>[3x]SNATLRIAAMPALANGLLPRFLAQFIRDRPNLQVSLMGL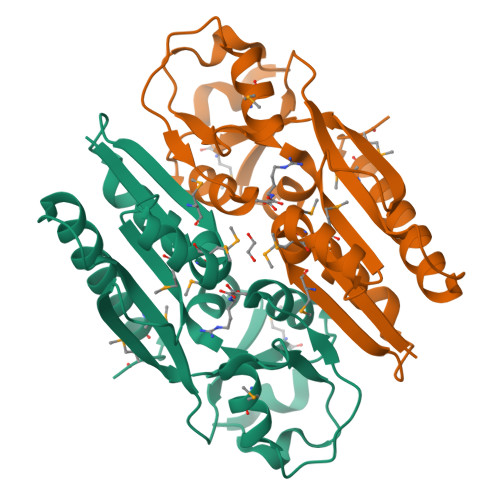PSSMVMEAVASGRADIGYADGPQERQGFLIETRSLPAVVAVPMGHRLAGLDRVTPQDLAGERIIKQETGTLFAMRVEVAIGGIQRRPSIEVSLSHTALSLVREGAGIAIIDPAAAIEFTDRIVLRPFSIFIDAEFLEVRSAIGAPSTIVDRFTTEFWRFHDDLMKQNGLME>[2x]LLPILSFPDPRLRTIAKPVEEVTDEIRQLAADMFETMYAAPGIGLAASQVDRHIQLIVMDLSESKDEPMVF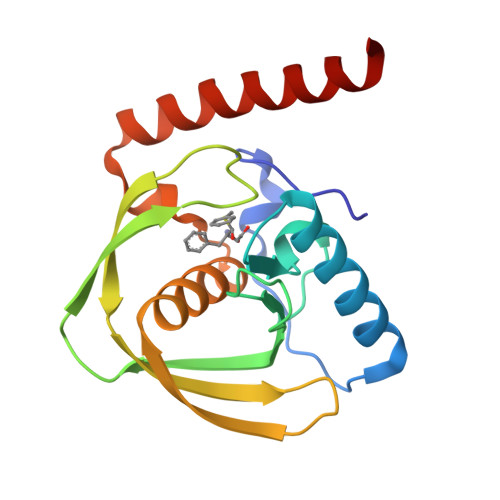INPKVTPLTEETQPYEEGCLSVPQIYDKVDRPSRVKIEAINLEGQAFEIEADGLLAVCIQHEMDHLNGKLFVDYLSPLKRQRAREKVEKIVRQREREKVA In mammals, NAD+ synthesis is largely dependent on the nicotinamide salvage pathway, in which NAMPT is the rate-limiting enzyme. NAMPT affects tumor cell proliferation and differentiation by participating in the NAD+ salvage pathway. As an important cofactor, NAD+ is involved in numerous life processes, including cellular energy metabolism, DNA transcription and repair, and redox homeostasis. Therefore, NAMPT is closely associated with tumor development.

(13aS)-3-Hydroxyl-6,7-dimethoxyphenanthro[9,10-b] indolizidine (PF403), a phenanthroindolizidine alkaloid, has been identified as a promising therapeutic agent for the treatment of glioma. In this study, we identified nicotinamide phosphoribosyl transferase (NAMPT) as the target of PF403 by using thermal proteome profiling (TPP). Moreover, microscale thermophoresis (MST), surface plasmon resonance (SPR), and isothermal titration calorimetry (ITC) experiments confirmed that NAMPT exhibits good affinity for PF403. Direct and indirect enzyme activity assays revealed that PF403 inhibited the catalytic activity of NAMPT, leading to a decrease in the concentration of nicotinamide adenine dinucleotide (NAD+) in U87 cells. Fortunately, we cultured and obtained a cocrystal of PF403 that is bound to NAMPT and found that PF403 binds to the rear channel of NAMPT active site. To explore the specific binding mode of the surrounding amino acids, we also performed an alanine scan and molecular dynamics simulation to identify potential key residues. These potential key amino acids were subsequently mutated, expressed, and purified through an E. coli system, followed by nanoDSF experiments. Finally, the pi–pi contacts and water–bridge interactions formed by Tyr188 were the keys to maintaining the binding of PF403 to NAMPT. Our research has identified a promising lead as an NAMPT binding agent for treating gliomas and revealed the precise interaction mode of the NAMPT–PF403 complex by X-ray diffraction. After NAMPT was knocked down with lentivirus, PF403 lost or partially lost its antitumor activity at the cellular and animal levels. These findings suggest that PF403 exerts antitumor activity by directly targeting NAMPT.

>MNPAAEAEFNILLATDSYKVTHYKQYPPNTSKVYSYFECREKKTENSKLRKVKYEETVFYGLQYILNKYLKGKVVTKEKIQEAKDVYKEHFQDDVFNEKGWNYILEKYDGHLPIEIKAVPEGFVIPRGNVLFTVENTDPECYWLTNWIETILVQSWYPITVATNSREQKKILAKYLLETSGNLDGLEYKLHDFGYRGVSSQETAGIGASAHLVNFKGTDTVAGLALIKKYYGTKDPVPGYSVPAAEHSTITAWGKDHEKDAFEHIVTQFSSVPVSVVSDSYDIYNACEKIWGEDLRHLIVSRSTQAPLIIRPDSGNPLDTVLKVLEILGKKFPVTENSKGYKLLPPYLRVIQGDGVDINTLQEIVEGMKQKMWSIENIAFGSGGGLLQKLTRDLLNCSFKCSYVVTNGLGINVFKDPVADPNKRSKKGRLSLHRTPAGNFVTLEEGKGDLEEYGQDLLHTVFKNGKVTKSYSFDEIRKNAQLNIELEAAHH[2x]> GAMGSMDSNTVSSFQVDCFLWHVRKQVADQELGDAPFLDRLRADQASLKGRGSTLGLNIETATCV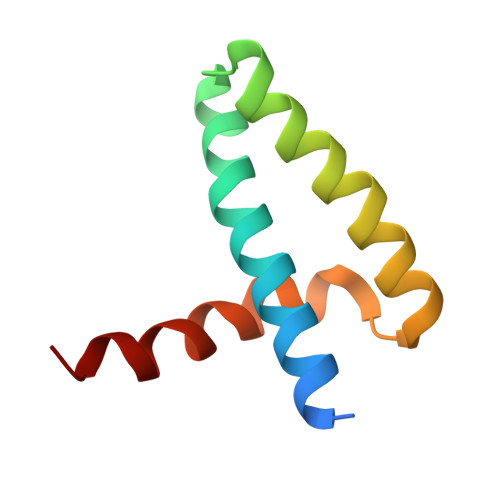GKQIVERILKEE>MVIASVEDGGDGDTSKDDWLWYKQPASQTDATATAGGNYGNPDNNRWQQTTLPFGNGKIGGTVWGEVSRERVTFNEETLWTGGPGSSTSYNGGNNETKGQNGATLRALNKQLANGAETVNPGNLTGGENAAEQGNYLNWGDIYLDYGFNDTTVTEYRRDLNLSKGKADVTFKHDGVTYTREYFASNPDNVMVARLTASKAGKLNFNVSMPTNTNYSKTGETTTVKGDTLTVKGALGNNGLLYNSQIKVVLDNGEGTLSEGSDGASLKVSDAKAVTLYIAAATDYKQKYPSYRTGETAAEVNTRVAKVVQDAANKGYTAVKKAHIDDHSAIYDRVKIDLGQSGHSSDGAVATDALLKAYQRGSATTAQKRELETLVYKYGRYLTIGSSRENSQLPSNLQGIWSVTAGDNAHGNTPWGSDFHMNVNLQMNYWPTYSANMGELAEPLIEYVEGLVKPGRVTAKVYAGAETTNPETTPIGEGEGYMAHTENTAYGWTAPGQSFSWGWSPAAVPWILQNVYEAYEYSGDPALLDRVYALLKEESHFYVNYMLHKAGSSSGDRL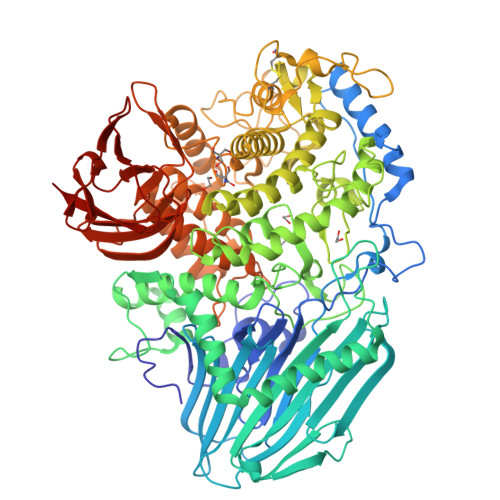TTGVAYSPEQGPLGTDGNTYESSLVWQMLNDAIEAAKAKGDPDGLVGNTTDCSADNWAKNDSGNFTDANANRSWSCAKSLLKPIEVGDSGQIKEWYFEGALGKKKDGSTISGYQADNQHRHMSHLLGLFPGDLITIDNSEYMDAAKTSLRYRCFKGNVLQSNTGWAIGQRINSWARTGDGNTTYQLVELQLKNAMYANLFDYHAPFQIDGNFGNTSGVDEMLLQSNSTFTDTAGKKYVNYTNILPALPDAWAGGSVSGLVARGNFTVGTTWKNGKATEVRLTSNKGKQAAVKITAGGAQNYEVKNGDTAVNAKVVTNADGASLLVFDTTAGTTYTITKKAS[2x]> SNAEEERIERWVEQLREALIGDGFLLHYQPVLNLQGEPLELYQAFLRLERNGEMMSPNAFMAIAEEHDLITEIDRWVVARAIRQLGERQRAGHKTHLLVRIGPNSFSDPQMIDTIREQLAVYGVPGERLWLQTPESKVFTHLRNAQQFLASVSAMGCKVGLEQFGSGLDSFQLLAHFQPAFLKLDRSITGDIASARESQEKIREITSRAQPTGILTVAEFVADAQSMSSFFTAGVDYVQGDFV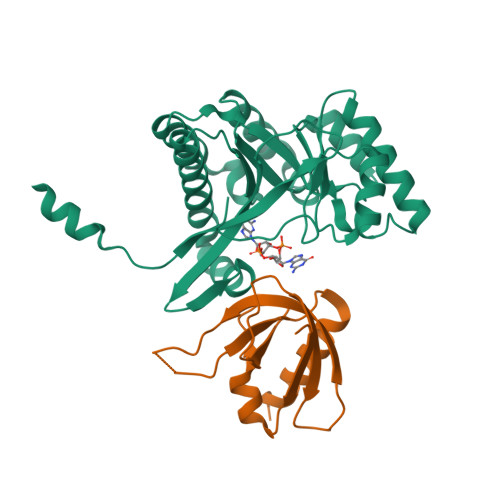APTGPLM;> MSAMNARQGILSLALKDKAALYSAYMPFVKSGGIFVPTPKRYMLGDEVFLLLTLPDSSERLPVAGKVVWTTPAGAQGNRAAGIGVQFPDGPEGEAVRNKIETLLAGLTTSDKPTHTM>AMELIRIAMKKDLENDNSLMNKWATVAGLKNPNPLYDFLNHDGKTFNEFSSIVNIVKSQYPDREYELMKDYCLNLDVKTKAARSALEYADANMFFEIEDALIDSMISCSNMKSKEYGKVYKIHRELSKGEIDVFEASANIGKQRIKTAEMNIFSKMLLMYDCLNKGNFAPMMLLFQQIDLSEIKENRYLKNSFETRINVLLSNIYLNENNLELCREYAQKAISSTDTQRFLVFSYLTIGTSYIFSDFNLSKQNYLIGLKFAKGNPGFEEFFKRNLSFLNNFWNKENEWINYDSDAVTDMQEVIFELINHKELSKALQLLNKLEERDQNENELGFHYYLKGLITNEKEAFFKSVEYFKASQDKLSIKMPLIQLEKMGENPRLLKIITM[2x];>[2x]GIVRGA

The arbitrium system is employed by phages of the SPbeta family to communicate with their progeny during infection to decide either to follow the lytic or the lysogenic cycle. The system is controlled by a peptide, AimP, that binds to the regulator AimR, inhibiting its DNA-binding activity and expression of aimX. AimR is a transcription factor that in its apo peptide-free form promotes aimX expression. In this study, we deepen our understanding of the system by solving the structure of an additional AimR that shows chimerical characteristics with the SPβ receptor.

The AimR-AimPKat asymmetric unit contains two AimR molecules arranged as a dimer, with one AimPKat bound to the TPR domain of each AimRKat protomer. The dimeric organisation in solution for the AimR-AimPKat complex was confirmed by SEC-MALS. Having the structures of AimRKat in its apo and AimPKat-bound conformations, we not only analysed the mechanism of peptide action but also whether it corresponds to any of the two alternative mechanisms proposed for AimRSPβ. This comparison showed that the peptide induces a closure movement of AimR protomer, produced by a ~15° relative rotation in the TPRN-ter subdomain (calculated with Dyndom15). Further, due to the reduced proximity of the subdomains, new interactions are produced between TPRN-ter and TPRC-ter that tie the protomer in the compact conformation. The distance between the DNA recognition helices (α3) in the AimR-AimPKat dimer is only 60 Å, a reduction of more than 20 Å in comparison to the apo AimRKat form. This separation between the two DBDs and their relative disposition is too small to allow them to interact with the two palindromic sequences present in the AimR operator which are separated ∼85 Å due to the 25 bp spacer, as confirmed by the superimposition of AimRKat and AimR-AimPKat in the structure of AimRSPβ bound to its DNA operator. In the AimR-AimPKat structure, the peptide binds to the concave side of the channel formed by the TPR-like repeats, and it establishes hydrophilic interactions at both N- and C-terminal ends, anchoring AimPKat in an extended conformation. The AimPKat N-terminal is bound to AimRKat Q299 and E300 side chains (TPR7) by a hydrogen bond and a salt bridge, respectively. AimRKat has an Asn at position 273 (N273) that anchors AimPKat V3 by interacting with its N and O backbone.>[6x]MDINASRALANVYDLPDDFFPKIDDLVRDAKDALEPYWKSDSIKKHVLIATHFVDLIEDFWQTTQGMHEIAESLRAVIPPTTTPVPPGYLIQHEEAEEIPLGDLFKHQEERIVSFQPDYPITARIHAHLKAYAKINEESLDRARRLLWWHYNCLLWGEAQVTNYISRLRTWLSTPEKYRGRDAPTIEAITRPIQVAQGGRKTTTGTRKPRGLEPRRRKVKTTVVYGRRRSKSRERRA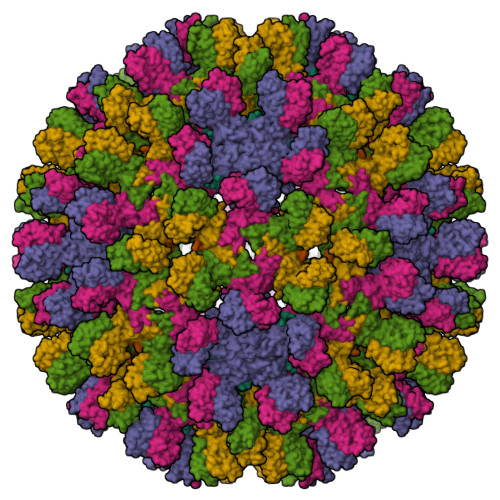PTPQRAGSPLPRSSSSHHRSPSPRK>[3x]VMTMRGLLVGRMQPFHRGHLQVIKSILEEVDELIICIGSAQLSHSIEDPFTAGERVMMLTKALSENGIPASRYYIIP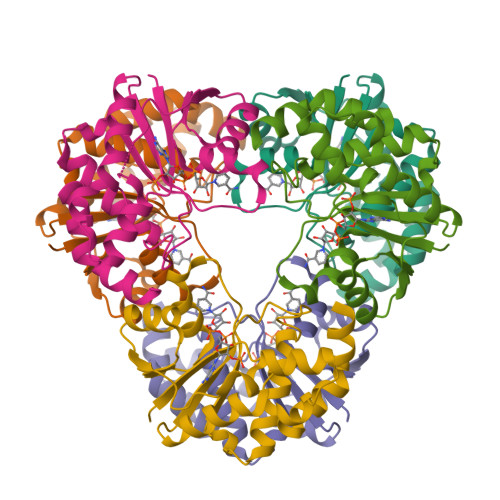VQDIECNALWVGHIKMLTPPFDRVYSGNPLVQRLFSEDGYEVTAPPLFYRDRYSGTEVRRRMLDDGDWRSLLPESVVEVIDEINGVERIKHLAKKEVSELGGIS> MDPLCAAPCSCDGDRRVDCSGKGLTAVPEGLSAFTQALDISMNNITQLPEGAFKNFPFLEELQLAGNDLSFIHPKALSGLKELKVLTLQNNQLKTVPSEAIRGLSALQSLRLDANHITSVPEDSFEGLVQLRHLWL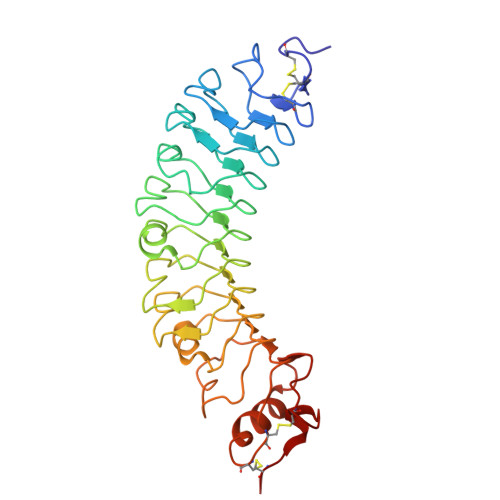DDNSLTEVPVHPLSNLPTLQALTLALNKISSIPDFAFTNLSSLVVLHLHNNKIRSLSQHCFDGLDNLETLDLNYNNLGEFPQAIKALPSLKELALDTNQLKSVPDGIFDRLTSLQKIWLHTNPWDCSCPRIDYLSRWLNKNSQKEQGSAKCSGSGKPVRSIICPT>[2x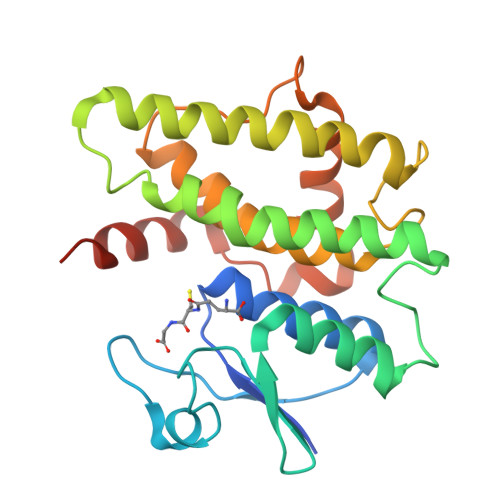]HHHHHHMAKSDVKLLGAWPSPFVMRPRIALNIKSVEYEFLEETLGSKSQLLLESNPVHKKIPVLIHGGKPICESLVIVEYIDEVWSPGPAILPSDPYDRALARFWAAYLDEKWFPTMRNIAAAKDEEARKALIDQVGEGLVLLEDAFSKCSKGKGFFGGDQIGYLDIAFGSFLGWLRAIEKMNGVKLMDETRTPGLLKWANSFSSHPAVKDVFPETEKLVEFAKVLAKLKATPPK>[4x]GSNRSLIVTTLLEEPFVMFRKSDRTLYGNDRFEGYCIDLLKELAHILGFSYEIRLVEDGKYGAQDDKGQWNGMVKELIDHKADLA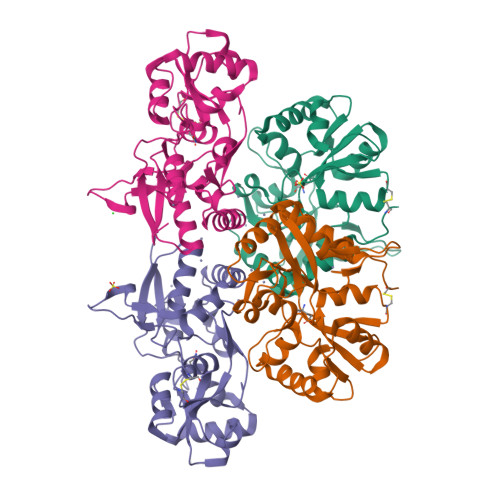VAPLTITHVREKAIDFSKPFMTLGVSILYRKGTPIDSADDLAKQTKIEYGAVKDGATMTFFKKSKISTFEKMWAFMSSKPSALVKNNEEGIQRTLTADYALLMESTTIEYITQRNCNLTQIGGLIDSKGYGIGTPMGSPYRDKITIAILQLQEEDKLHIMKEKWWRGSGCPE>GSENLYFQSGSMARQERAIRTRQTILVAAAEVFDEVGYEAATISDVLKRSGVTKGALYFHFTSKQELAQAVLAEQVASLPRVPEQELKLQQSLDEALLLAHLLREGTGDPIVQGSVRLTVDQGSPRDHLNRRVPMQAWTEHTQSLFEEARAKGEI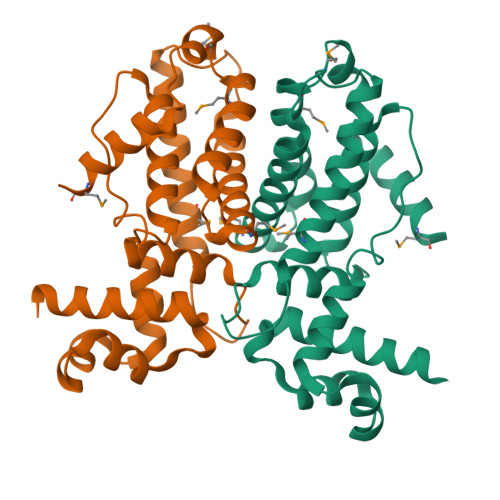LPHADVEALAKLFVGAFTGVQVLSRIMTGRADLAERVADLYRHLMPSFAMPGILVRLDFSPERGSRVYEAAMKQRESAAASTTDAARTLE[4x]>[2x]GMYAVPILNVYDFEVKKDKETSYKSATEDYVNKTMGVEQGVLGLFAATDERDKTTSYIVEIYN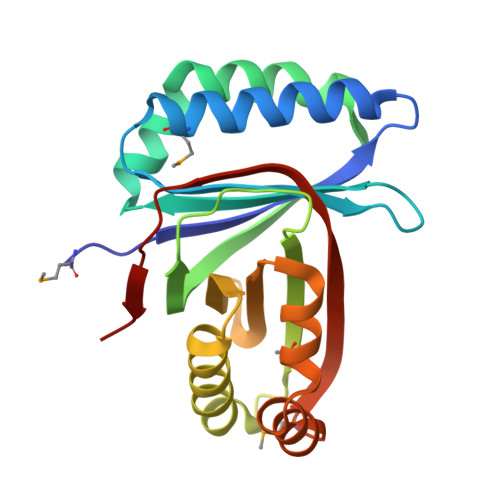DYLAFSNHTKNQASKDFKAVIPQIAEGNLNSAEIDVQIAKDKKIEQNDNTFAVYTVIDVKPENDKEFAEIIKNIVETTFNEEGTLLVYLGTDRRNFNKWCLFEVYKDIDSYLNHRSAKYFKDYITQTKDMIAGKKRAELQVLKIENKGGLDYKKLY> ISGGDAIYSSTGRCSLGFNVRSGSTYYFLTAGHCTDGATTWWANSARTTVLGTTSGSSFPNNDYGIVRYTNTTIPKDGTVGGQDITSAANATVGMAVTRRGSTTGTHSGSVTALNATVNYGGGDVVYGMIRTNVCAEPGDSGGPLYSGTRAIGLTSGGSGNCSSGGTTFFQPVTEALSAYGVSVY;> VDCSEYPK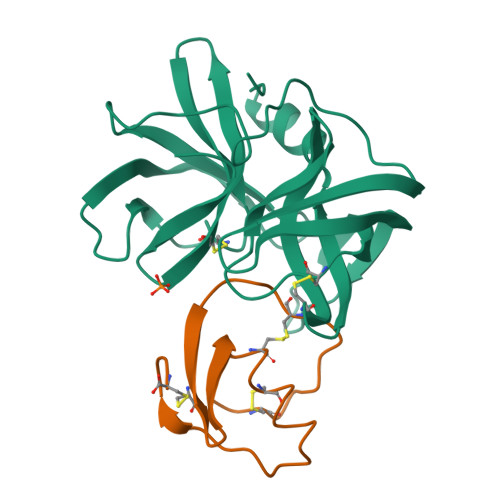PACTNEYRPLCGSDNKTYGNKCNFCNAVVESNGTLTLSHFGKC>[2x]TLTKHEQDILLKELGPHVDTPAHIVETGLGAYHALFTAHPQYISHFSRLEGHTIENVMQSEGIKHYARTLTEAIVHMLKEISNDAEVKKIAAQYGKD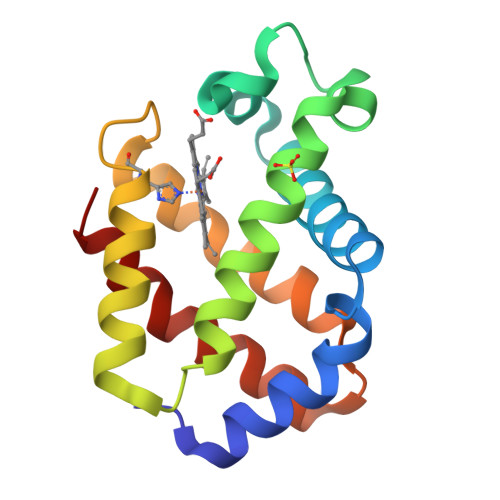HTSRKVTKDEFMSGEPIFTKYFQNLVKDAEGKAAVEKFLKHVFPMMAAEI TRIMETREXATE | C19 H24 N5 O3 | 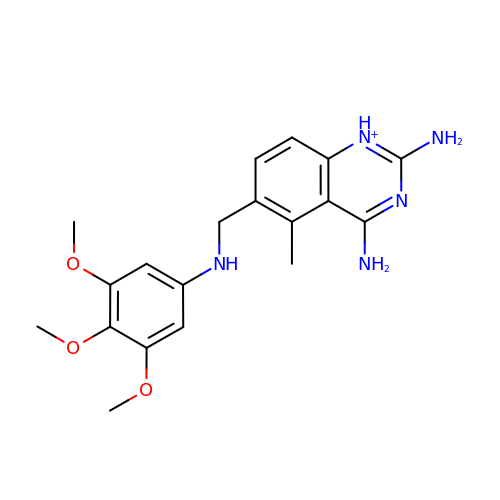NOYPYLRCIDNJJB-UHFFFAOYSA-O> MGLIFAKLWSLFCNQEHKVIIVGLDNAGKTTILYQFLMNEVVHTSP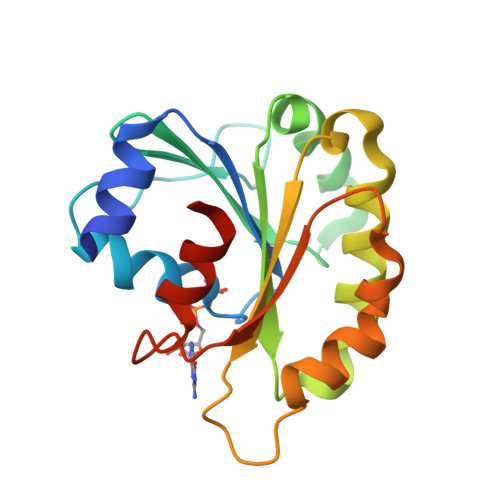TIGSNVEEIVVKNTHFLMWDIGGQESLRSSWNTYYSNTEFIILVVDSIDRERLAITKEELYRMLAHEDLRKAAVLIFANKQDMKGCMTAAEISKYLTLSSIKDHPWHIQSCCALTGEGLCQGLEWMTSRIGVR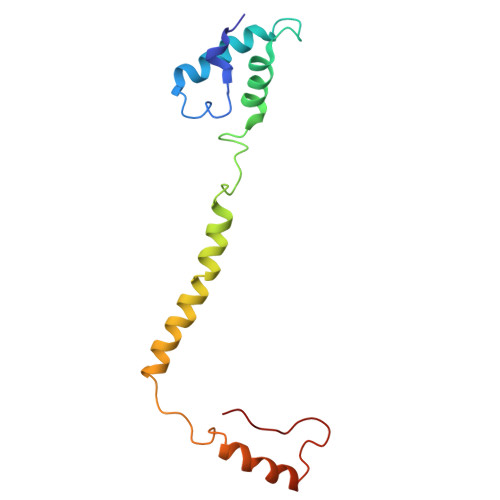> ALSNAAVMDLQSRWENMPSTEQQDIVSKLSERQKLPWAQLTEPEKQAVWYISYGEWGPRRPVLNKGDSSFIAKGVAAGLLFSVGLFAVVRMAGGQDAKTMNKEWQLKSDEYLKSKNANPWGGYSQVQS> SSMEIRVRVEKDPELGFSISGGVGGRGNPFRPDD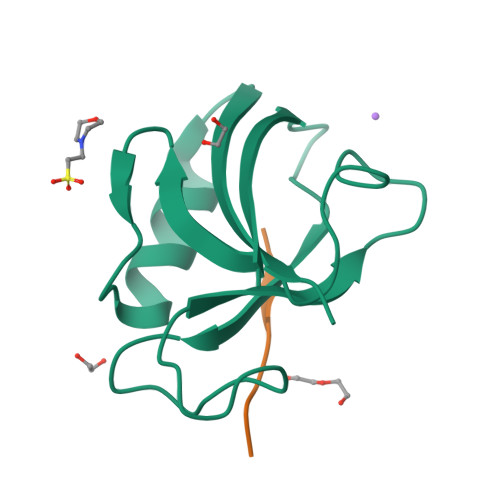DGIFVTRVQPEGPASKLLQPGDKIIQANGYSFINIRLEEAERLLKTFQNTVELIIVREVSS;> RWYERWV>[2x]APTAKLANGDTITGLNAIINEAFLGIPFAEPPVGNLRFKDPVPYSGSLNGQKFTSYGPSCMQQNPEGTFEENLGKTALDLVMQSKVFQAVLPQSEDCLTINVVRPPGTKAGANLPVMLWIFGGGFEIGSPTIFPPAQMVTKSVLMGKPIIHVAVNYRVASWGFLAGDDIKAEGSGNAGLKDQRLGMQWVADNIAGFGGDPSKVTIFGESAGSMSVLCHLIWNDGDNTYKGKPLFRAGIMQSGAMVPSDPVDGTYGNEIYDLFVSSAGCGSASDKLACLRSASSDTLLDATNNTPGFLAYSSLRLSYLPRPDGKNITDDMYKLVRDGKYASVPVIIGDQNDEGTVFGLSSLNVTTNAQARAYFKQSFIHASDAEIDTLMAAYPQDITQGSPFDTGIFNAITPQFKRISAVLGDLAFIHARRYFLNHFQGGTKYSFLSKQLSGLPIMGTFHANDIVWQDYLLGSGSVIYNNAFIAFATDLDPNTAGLLVNWP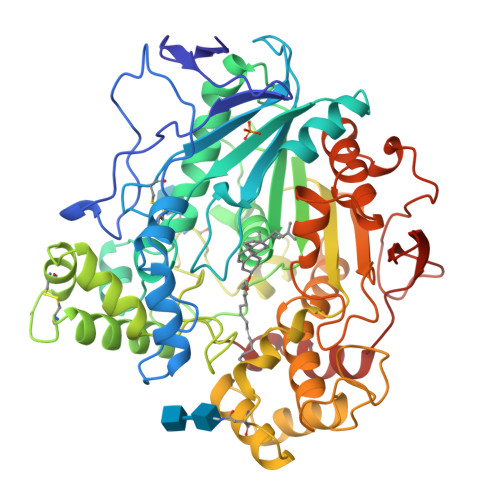KYTSSSQSGNNLMMINALGLYTGKDNFRTAGYDALMTNPSSFFV> GAMGSTSLEPTSTLVRVRKSAATLGIAI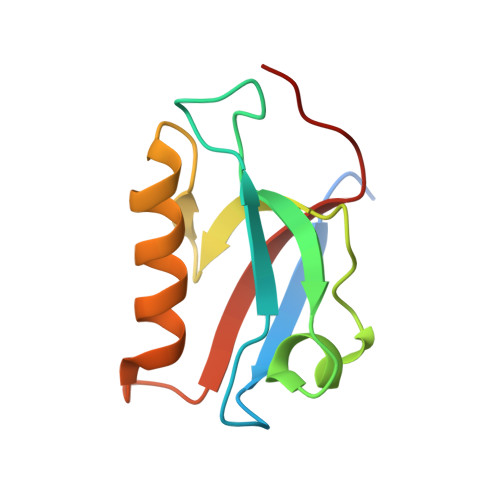EGGANTRQPLPRIVTIQRGGSAHNCGQLKVGHVILEVNGQTLRGKEHKEAARIIAEAFKTKERDYIDFLVTEFNVML>MARYDKYNPYGGGFRAPLAADWTDADAGKLYAVGINNVGAVVKGAGQSGVAGVLVLTKGAKAGSIVDVMKFGEVVEFGPTSGTPGTDFGAAGTAYYADTSTGAINSTSGEAKVKVGHTVGAQRLIVAVADGVVDPSPAA[7x];>MKTATEGRVMRESFLEIIAVVGLSGHDNQGGYNTAGDIKYKTADGVSYDSLWNLFSNVTDEWNKHKSKMVQLMTFPVTNQTEKVPRIGQFGFEKASEFGVPESKRTELSFYQLAYD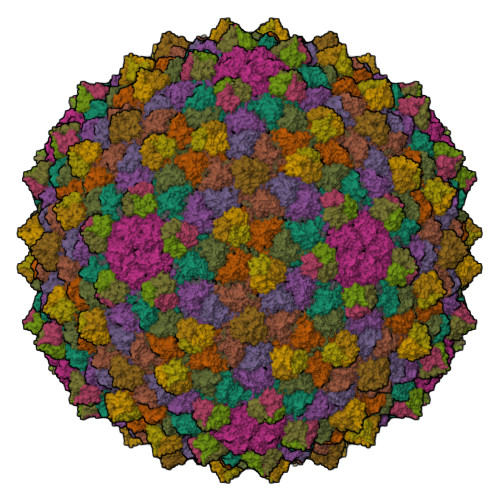FEDYDLAFRYTWKFLRDAPSSQIKAYHNQALQADAKLIHRKVMEAIFDNREREADIEGLPYKVYPLYNGDNMIPPEYNGTTFSTGHNHYLVSGGTKIDSADVEMAADHIREHGYTEENGTQLIAFAHKAEIQEVRRFRFGQTNNNSAVANYDFVQSQGESPLYLPNADGLLGKQPQSMWKGLRVKGSYDDVLWIEEPTMPAGYVLFLATGGTLAQQNLVGLREHEDAAWRGLRQIPGNQTRYPLIDSFYQRSFGTGIRQRGGAVVLQIKASGTYDIPTKWTNGGGFE[7x];>MAKGVKKLPKRKGTNPIPRDKWNSDDIARRQLEQDQKLHLTTKGPHTGTNDSFK[2x]> MSLSDLSAFAVTQKWPAQFPEWIQLYSLPTPNGVKVSIMLEEIGLPY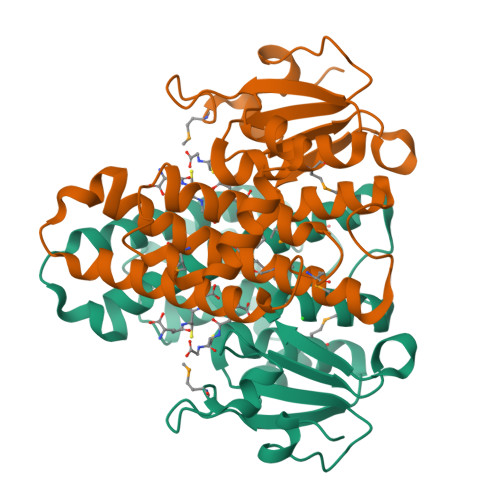EAHRVSFETQDQMTPEFLSVSPNNKIPAILDPHGPGDQPLALFESGAILIYLADKSGQLLAQESAARYETIQWLMFQMGGIGPMFGQVGFFNKFAGREYEDKRPLERYVNEAKRLLGVLDKHLGGREWIMGERYTIADIATFPWIRNLIGFYEAGELVGIDNFPEVKRVLAKFVARPAVIRGLEIPKVSEGHHHHHH N-[4-[(5R)-6-oxidanylidene-5-quinolin-5-yl-5-(trifluoromethyl)-1,4-dihydropyridazin-3-yl]phenyl]-1,3-dihydropyrrolo[3,4-c]pyridine-2-carboxamide | C28 H21 F3 N6 O2 | 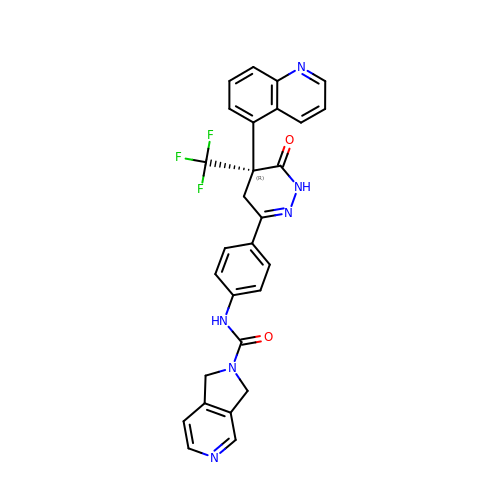KQAUKAZYPSSEKR-HHHXNRCGSA-N> GSHMASPNGQTKPLPALKLALEYIVPCMNKHGICVVDDFLGKETGQQIGDEVRALHDTGKFTDGQLVSQKSDSSKDIRGDKI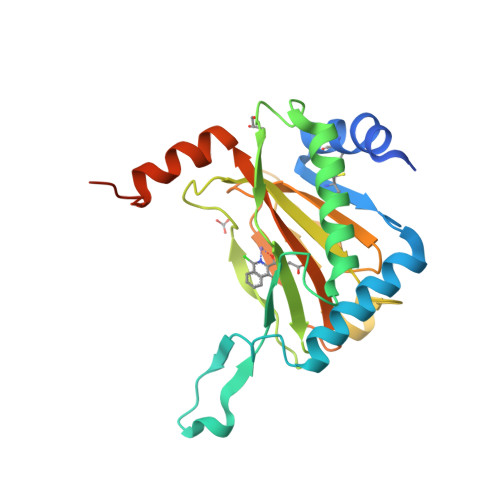TWIEGKEPGCETIGLLMSSMDDLIRHCNGKLGSYKINGRTKAMVACYPGNGTGYVRHVDNRNGDGRCVTCIYYLNKDWDAKVSGGILRIFPEGKAQFADIEPKFDRLLFFWSDRRNPHEVQPAYATRYAITVWYFDADERARAKVKYLTGEKGVRVELNKPSDSVGKDVF> GPLGSPGSRAMA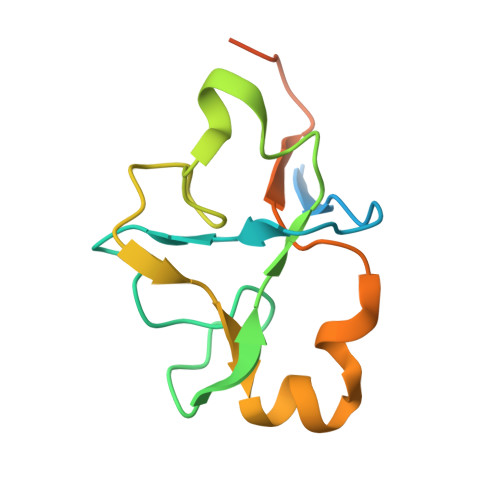KHHPDLIFCRKQAGVAIGRLCEKCDGKCVICDSYVRPCTLVRICDECNYGSYQGRCVICGGPGVSDAYYCKECTIQEKDRDGCPKIVNLGSSKTDLFYERKKYGFKKR2-({[4-(TRIFLUOROMETHOXY)PHENYL]SULFONYL}AMINO)ETHYL DIHYDROGEN PHOSPHATE | C9 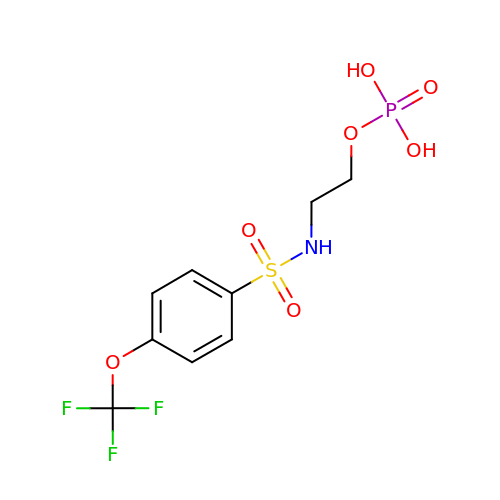H11 F3 N O7 P S | JDDKDMFCTOZVCJ-UHFFFAOYSA-N>[2x]MNHKVHMKNIQVVVRCRPFNLAERKASAHSIVECDPVRKEVSVRTGGLADKSSRKTYTFDMVFGASTKQIDVYRSVVCPILDEVIMGYNCTIFAYGQTGTGKTFTMEGERSPNEEYTWEEDPLAGIIPRTLHQIFEKLTDNGTEFSVKV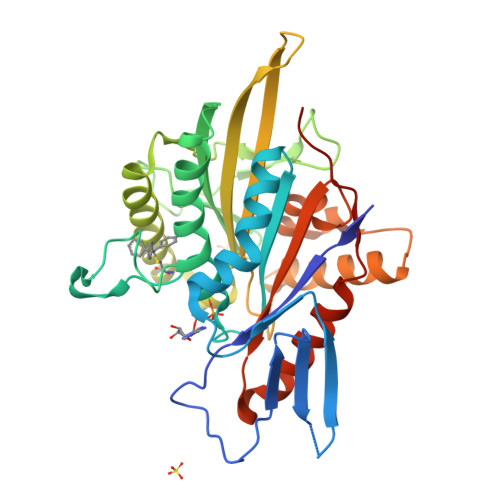SLLEIYNEELFDLLNPSSDVSERLQMFDDPRNKRGVIIKGLEEITVHNKDEVYQILEKGAAKRTTAATLMNAYSSRSHSVFSVTIHMKETTIDGEELVKIGKLNLVDLAGSENIGRSGAVDKRAREAGNINQSLLTLGRVITALVERTPHVPYRESKLTRILQDSLGGRTRTSIIATISPASLNLEETLSTLEYAHRAKNILNKPEVNQKLQHHHHHH>[2x]EFNILLATDSYKVTHYKQYPPNTSKVYSYFECREKKT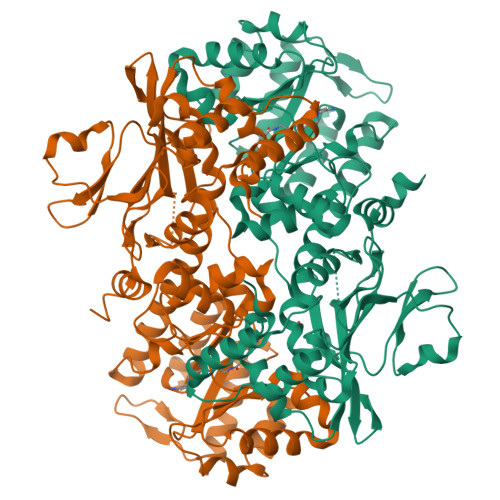ENSKLRKVKYEETVFYGLQYILNKYLKGKVVTKEKIQEAKDVYKEHFQDDVFNEKGWNYILEKYDGHLPIEIKAVPEGFVIPRGNVLFTVENTDPECYWLTNWIETILVQSWYPITVATNSREQKKILAKYLLETSGNLDGLEYKLHDFGYRGVSSQETAGIGASAHLVNFKGTDTVAGLALIKKYYGTKDPVPGYSVPAAEHSTITAWGKDHEKDAFEHIVTQFSSVPVSVVSDSYDIYNACEKIWGEDLRHLIVSRSTQAPLIIRPDSGNPLDTVLKVLEILGKKFPVTENSKGYKLLPPYLRVIQGDGVDINTLQEIVEGMKQKMWSIENIAFGSGGGLLQKLTRDLLNCSFKCSYVVTNGLGINVFKDPVADPNKRSKKGRLSLHRTPAGNFVTLEEGKGDLEEYGQDLLHTVFKNGKVTKSYSFDEIRKNAQLNIELE> MSLTNHTETITVEEGQTLTLKCVTSLRKNSSLQWLTPSGFT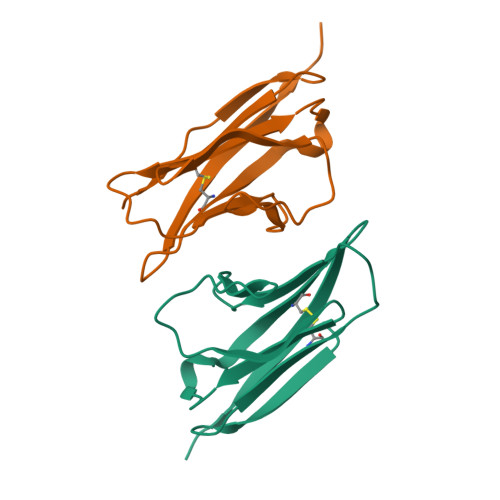IFLNEYPALKNSKYQLLHHSANQLSITVPNVTLQDEGVYKCLHYSDSVSTKEVKVIVLAT;> MQNLFTKDVTVIEGEVATISCQVNKSDDSVIQLLNPNRQTIYFRDFRPLKDSRFQLLNFSSSELKVSLTNVSISDEGRYFCQLYTDPPQESYTTITVLVPP>GSFVEMVDNLRGKSGQGYYVEMTVGSPPQTLNILVDTGSSNFAVGAAPHPFLHRYYQRQLSSTYRDLRKGVYVPYTQGKWEGELGTDLVSIPHGPNVTVRANIAAITESDKFFINGSNWEGILGLAYAEIARPDDSLEPFFDSLVKQTHVPNLFSLQLCGAGFPLNQSEVLASVGGSMIIGGIDHSLYTGSLWYTPIRREWYYEVIIVRVEINGQDLKMDCKEYNYDKSIVDSGTTNLRLPKKVFEAAVKSIKAASSTEKFPDGFWLGEQLVCWQAGTTPWNIFPVISLYLMGEVTNQSFRITILPQQYLRPVEDVATSQDDCYKFA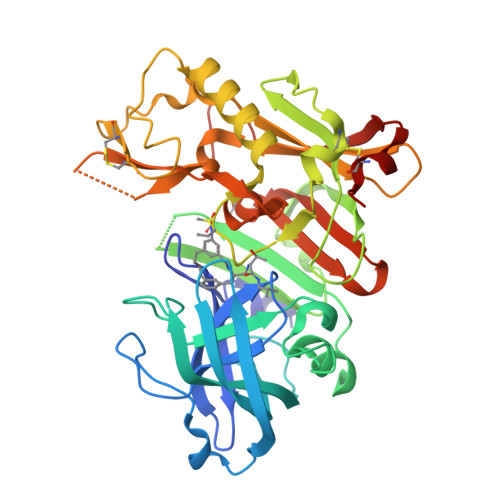ISQSSTGTVMGAVIMEGFYVVFDRARKRIGFAVSACHVHDEFRTAAVEGPFVTLDMEDCGYNI[3x]> GAMASNSEILKYATEEEKKILIPILRKKPVRTISGVAVVAVMTSPAKCPHGKCIFCPGGLDSVFGDVPQSYTGREPATMRGLMFNFDPYLQTRARIEQLEKVGHPTDKIELIIMGGTFPAREIEYQDWFIKRCLDAMNERESKSLEEAQKINETAKHRCVALCIETRPDYCSEKEINQMLKLGATRVELGVQSIYNEILKLCKRGHSVEDTIKATQLLKDSGLKVSYHLMPGMPGSSIEMDKKMFKEIFTNPDFMPDMVKIYPCLVIEGTELYEMWKRGEFKPYREEEAIEVISYAKSIMPKWVRTSRIQRDIPATVIVDGVKKSNLGELVYKYMEKKGLRCRCIRCREVGHVYYKKGILPDPEHIKLVREDYEASGGTEIFLSFEDVKNDILIAFLRLRDPYKPFRKEIDDK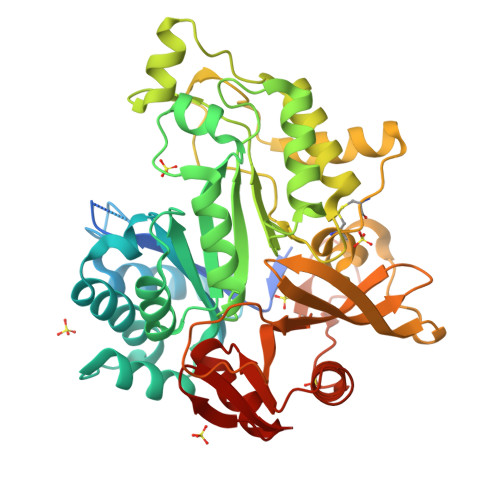TMLVRQLHVFGWEKALTRDIKEVSWQHMGYGRMLMKEAERIAKEEFGKKKILVTSGIGVREYYRKLGYKRVGAYMGKEL>MSLRITRLTVFHLDLPLAKPYWLSGGRLKFDRLDSTYLRIDTDEGVTGWGEGCPWGHSYLPAHGPGLRAGIATLAPHLLGLDPRSLDHVNRVMDLQLPGHSYVKSPIDMACWDILGQVAGLPLWQLLGGEAATPVPINSSISTGTPDQMLGLIAEAAAQGYRTHSAKIGGSDPAQDIARIEAISAGLPDGHRVTFDVNRAWTPAIAVEVLNSVRARDWIEQPCQTLDQCAHVARRVANPIMLDECLHEFSDHLAAWSRGACEGVKIKPNRVGGLTRARQIRDFGVSVGWQMHIEDVGGTALADTAALHLAAS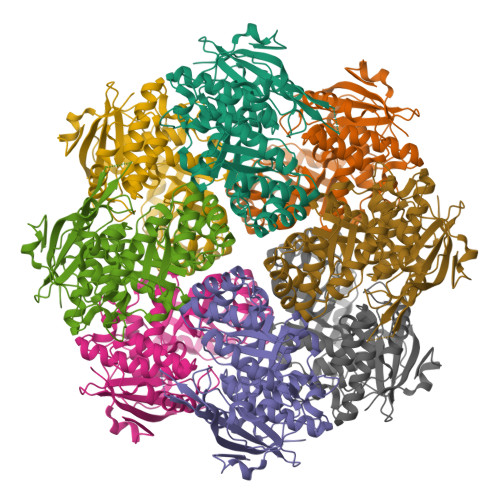TPEANRLASWLGHAHLADDPIPGQGARNRDGLATPPSAPGLGVIPDPEALGRPVASYDEGHHHHHH[2x]>[4x]HCHQQLNSLPTMEG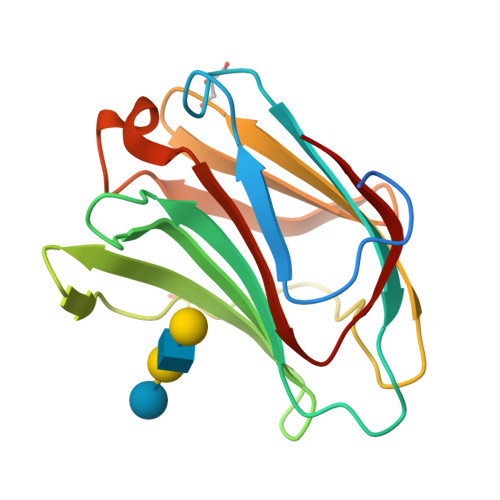PPTFNPPVPYFGRLQGGLTARRTIIIKGYVPPTGKSFAINFKVGSSGDIALHINPRMGNGTVVRNSLLNGSWGSEEKKITHNPFGPGQFFDLSIRCGLDRFKVYANGQHLFDFAHRLSAFQRVDTLEIQGDVTLSYVQI>GPSFWLGNETLKVPLALFALNRQRLCERLRKNPAVQAGSIVVLQGGEETQRYCTDTGVLFRQESFFHWAFGVTEPGCYGVIDVDTGKSTLFVPRLPASHATWMGKIHSKEHFKEKYAVDDVQYVDEIASVLTSQKPSVLLTLRGVNTDSGSVCREASFDGISKFEVNNTILHPEIVECRVFKTDMELEVLRYTNKISSEAHREVMKAVKVGMKEYELESLFEHYCYSRGGMRHSSYTCICGSGENSAVLHYGHAGAPNDRTIQNGDMCLFDMGGEYYCF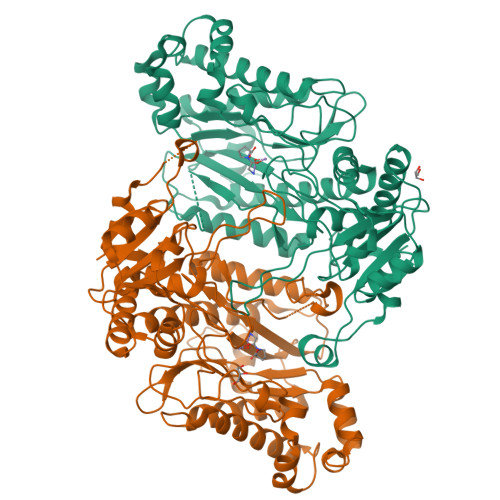ASDITCSFPANGKFTADQKAVYEAVLRSSRAVMGAMKPGVWWPDMHRLADRIHLEELAHMGILSGSVDAMVQAHLGAVFMPHGLGHFLGIDVHDVGGYPEGVERIDEPGLRSLRTARHLQPGMVLTVEPGIYFIDHLLDEALADPARASFLNREVLQRFRGFGRVRIEEDVVVTDSGIELLTCVPRTVEEIEACMAGCDKAFT[2x]>PYSLGPKISDWDEQRRDWLKQNPSFPNFVAPNKPRVLLVTGSAPKPCENPVGDHYLLKSIKNKIDYCRIHGIEIFYNMALLDAEMAGFWAKLPLIRKLLLSHPEIEFLWWMDSDAMFTDMVFELPWERYKDYNLVMHGWNEMVYDQKNWIGL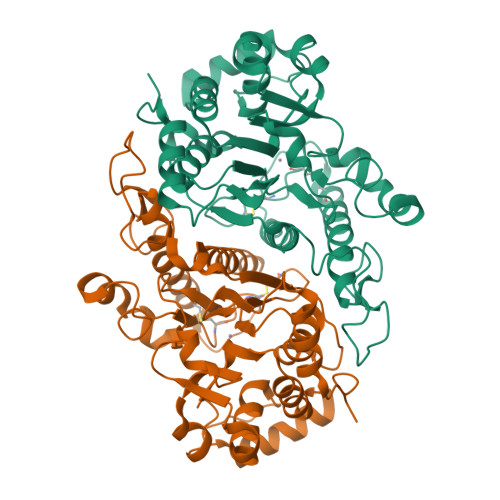NTGSFLLRNSQWSLDLLDAWAPMGPKGKIREEAGKVLTRELKDRPAFEADDQSAMVYLLATEREKWGGKVYLESGYYLHGYWGILVDRYEEMIENHKPGFGDHRWPLVTHFVGCKPCGKFGDYPVERCLRQMDRAFNFGDNQILQMYGFTHKSLGSRRVKPTRNQTDRPLDAKDEFGLLHPPFKAA[2x]The PfEMP1 family of surface proteins is central for Plasmodium falciparum virulence and must retain the ability to bind to host receptors while also diversifying to aid immune evasion. The interaction between CIDRα1 domains of PfEMP1 and endothelial protein C receptor (EPCR) is associated with severe childhood malaria. We combine crystal structures of CIDRα1:EPCR complexes with analysis of 885 CIDRα1 sequences, showing that the EPCR-binding surfaces of CIDRα1 domains are conserved in shape and bonding potential, despite dramatic sequence diversity. Additionally, these domains mimic features of the natural EPCR ligand and can block this ligand interaction.

Crystals of the HB3var03 CIDRα1.4:EPCR complex formed and diffracted to 2.65Å resolution. The structure was consistent with an envelope obtained from solution small-angle X-ray scattering, and the two copies of HB3var03 CIDRα1 in the asymmetric unit aligned with a root-mean-square deviation (rmsd) of just 0.09Å, showing them to be extremely similar. The HB3var03 CIDRα1:EPCR interface has a surface area of 978Å2 and surrounds the kinked helix. At its center is a small hydrophobic patch containing F656 and F655, which interact with a hydrophobic patch on EPCR. In particular, F656 is positioned at the bend in the kinked α helix, where it protrudes from the domain surface, allowing it to insert into the hydrophobic groove of EPCR. This patch lies within a larger surface that is complementary in shape to EPCR and contains a series of amino acids (D576, K642, D652, S653, Q657, Y660, and K661) that make hydrogen bonds to EPCR side chains. However, the F656A mutation, which removes the majority of this interaction, had a 35-fold effect on the affinity and significantly increased the off rate, with a 100-fold change in the dissociation rate constant. Therefore, the insertion of F656 into the hydrophobic groove of EPCR increases the lifetime of the complex. In particular, F4 binds to the same site as F656 from HB3var03 CIDRα1. The CIDRα1-binding site is larger than that of protein C, extending to make contacts with two additional EPCR loops (residues 22–25 and 44–47) through K642 of the HB3var03 CIDRα1 domain.

>[2x]PDCGVECKNETCTPKTVIYPDCGKNEKYEPPGDAKNTEINVINSGDKEGYIFEKLSEFCTNENNENGKNYEQWKCYYDNKKNNNKCKMEINIANSKLKNKVTSFDEFFDFWVRKLLIDTIKWETELTYCINNTDVTDCNKCNKNCVCFDKWVKQKEDEWTNIMKLFTNKHDIPKKYYLNINDLFDSFFFQVIYKFNEGEAKWNELKENLKKQIASSKANNGTKDSEAAIKVLFNHIKEIATICKDNNTNEG;>LQRLHMLQISYFRDPYHVWYQGNASLGGHLTHVLEGPDTNTTIIQLQPLQEPESWARTQSGLQSYLLQFHGLVRLVHQERTLAFPLTIRCFLGCELPPEGSRAHVFFEVAVNGSSFVSFRPERALWQADTQVTSGVVTFTLQQLNAYNRTRYELREFLEDTCVQYVQKHI[2x]4-[(2~{R},3~{a}~{S},5~{S},6~{S},6~{a}~{S})-6'-chloranyl-6-(3-chloranyl-2-fluoranyl-phenyl)-4-(cyclopropylmethyl)-2'-oxidanylidene-spiro[1,2,3,3~{a},6,6~{a}-hexahydropyrrolo[3,2-b]pyrrole-5,3'-1~{H}-indole]-2-yl]benzoic acid | C30 H26 Cl2 F N3 O3 | 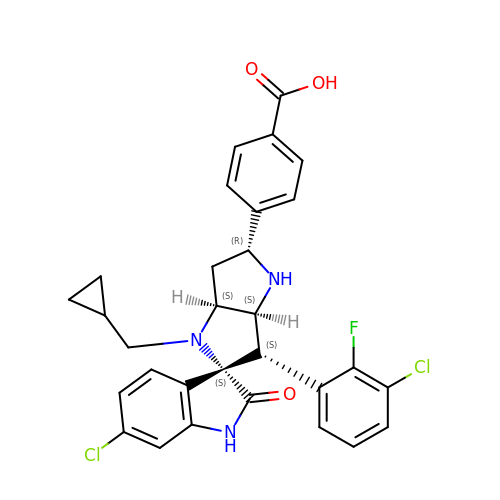CCPUFNJKOGKOOG-AFKAWQRRSA-N>MKVGIDAGGTLIKIVQEQDNQRTFKTELTKNIDQVVEWLNQQQIEKLCLTGGNAGVIAENINIPAQIFVEFDAASQGLGILLKEQGHDLADYIFANVGTGTSLHYFDGQSQRRVGGIGTGGGMIQGLGYLLSQITDYKQLTDMAQHGDRNTIDLKVRHIYKDTEPPIPGDLTAANFGHVLHHLDADFTPSNKLAAVIGVVGEVVTTMAITVAREFKTENIVY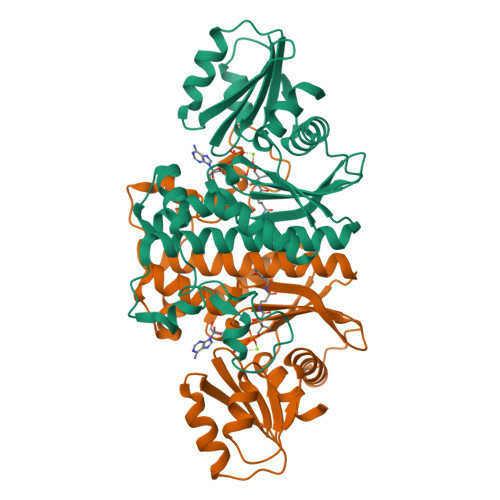IGSSFHNNALLRKVVEDYTVLRGCKPYYVENGAFSGAIGALYL[4x]Axonemal outer dynein arm (ODA) motors generate force for ciliary beating. Each HC of the axonemal dynein consists of an N‐terminal tail domain followed by the motor domain. This includes six AAA motifs (named AAA1–AAA6), with a microtubule‐binding domain (MTBD) connected to AAA4 by a coiled‐coil stalk, similar to its homolog cytoplasmic dynein. We analyzed three states of the ODA during the power stroke cycle using in situ cryo‐electron tomography, subtomogram averaging, and classification.

We thus have obtained an apo state, depicting the post‐PS conformation from a nucleotide‐free dataset. Our analysis shows that in the absence of ATP, all dynein linkers interact with the AAA3/AAA4 domains, indicating that interactions with the adjacent microtubule doublet B‐tubule direct dynein orientation. The tomographic map suggests that the γ linker is in a Post‐2 conformation, which was observed in neither MTBS1 nor MTBS2. In situ all three linkers appear to be in a Post‐2 conformation. MTBS1 fits worse than the MTBS2 model, which has the β and α homolog linker in a Post‐2 conformation. To optimize the fitting of the MTBS2 to the cryo‐ET map, we performed rigid body fitting and real‐space refinement of individual parts of the structure by Coot. Step 1 is the translation and rotation of the γ dynein head including the MTBD. The linker of the γ‐HC changes from a Post‐1 conformation to a Post‐2 conformation (Movie EV2). In addition, the stalk of the α‐HC adapts to a more straight conformation by a 1 nm distal movement of the MTBD. The resulting MTBS3 structure is shown in Fig 3F–M. Through this remodeling, the cross‐correlation score between the 20 Å filtered MTBS2 and MTBS3 structures and the cryo‐ET map increased from 0.6797 to 0.8402 (Movie EV3). In the post‐PS conformation, the stalks are upright and extended, maintaining a certain distance between two MTDs.

> MLSSKYSKRIAWMKTTICDSLQLKDMIVEESFQYEKNKNLLEQFLSGEGLNKIFAYYQVQEQAQNDDIKDTGAQDPVLFFTTGDLEKIQDKAVWFLRITNPADDKKKASQQDGNDNDIIFGEITPNTVPMLNALMESVYSRQIDHIITEKIQFWGVAEEEQVLEFQQHSNKFSSEVREAINLMSPGTEHFKLDYEAISGLSESEKMQHYEMKFNEWINLISSQLNDDSEVRKDEKDAGPATELIYWRSRMQKITNWSEQLKSKDFQIVKASLQRHKNHDNQRPRGDESLSKLMMEYNRLDLLLTDKLNEAKDNVKYLTTLEKFIEPLYNGTPQQIIDTLPALMNAIKMIHTIARFYNTTDKMTGLFIKITNQMIKNCKDRILNKKDNGDNPSLYKMIWEQDPAELIEVLGSCIKLYCEYKKCYNDTKEKVADMPKGKTFDFSDAQIFGKFDTFVRRLQKLIEIFSNIQQFNALAKHNLEGMDVLTNKFKKIIDDFKKKGHNLLDTANNKFDRDWVEFNVEISHLDGELQNFIDNNFNRFRNIEYSLKLLHKFQSTIKRDSLKHNLTSRYNAILHNYATELDTIQRVFQDQKSNPPLVRNMPPEAGKIIWARHLFQKITGPINIFPENVINSTEIRRYYGSYNTLGKQLTIYEMWFYQDWVNKIEQSKAALQATLIVRHDENKKLYVNFDLEIMQLIREAKCLDRQGIEIPESARIILLQEDKFKTYYNELLYALKEYERINSKIKPICKNLLLPHIEDLDLKLRPGMVTLTWTSMNIESYLYYVHQGLKKLEQLIINVNDIIENRIENNLKTVSKVVLVHLPQDTKPLSLDSFVQLQEEYINSKTDFLTSKNVEVERAVDDLLQTIMLYPLDPHVDPVLPEETKRIKRYYFWYFYQALLNSTQNSLNAMKYRVCGKKIPGANTLQNLKPFFQVEVQLNGDKVTLNPSLQEIQKSINRAATAVLRCSKHLYNWDQQNKDSTDKATFYDMIACDKEIVKVILLLTGSIQGTKNKVNEFLSGFTKFEWLCKESIQESIKKFSKNGPTLQNYEDQLKKFSQIEEEIEKIVPTYKIGAMELMTHNICTSLSTWAKEWKLQYSQDLHKRARQLLDSLTEQTKMLSTKLSKPVKDIDSLGYVMETLEQIRKEQAEIDMKFNPVQEMYSLLDNYLPGGITDKDEMDARSLLRRNWDILIQQAEIKGKEYQHKQAIYLKELKQSIKDFTNQVSIFRRDYEKNGPMVEGISPAEAMERLRRFEDEYDVKYQMYKINARGENLFGLQNQKYPELEKTDAEIKNLNKLYNLYDSVIKNIQQFKEKSWQDVSKDDLAKMEEDAGKYGEQCSRLPKDLKEWQAYRDLKNYIDSLREQLPLIISLKKPSIMPRHWEKIKEITNTKLNYENPDQFYIEEIMGAKLLDFREDIEDITESADKQLKIRTGLDEINLYWNDMQFQFGIWGKRDVPCMLNGLIVGTILERLEEDQLQLSTFNSQRHVTPFKAEVENLIRTFSDVNDTLDMWVKVQKLWTSLEPVFTGGDIARQMPLQAKQFQGIDKNWMKIMEKAVETKKVIPCCQNDMLKDFLPDLNRKLEDCQKMLEAYLEGKRKKFPRFYFVSNPTLLKILSQGSEPTSIQEDFEKLFDAITKVTFESAKDKKNPALKQITQIQQVIGRNEENISLTGYYVKCEGNIEDWLKKLEQNMQQTLKDIASAAAQQVFQVGLKEFVSSQASQIALLGLQILWTSKVNEGLERLSRNERNAMDIKRNEIKEHMNILSSMCLEDLNGAVERTKVETLVTIQVHQKDISMDLKCKDVNDFEWQKQTRIAWKTDIDECIISITDWDSPYSYEFLGAKERLCITPLTDRCYITLAQAMSMYYGGAPAGPAGTGKTETVKDLGRTLGVFVVVTNCSDQHRYRDMAKIFKGLVQSGLWGCFDEFNRIDLEVLSVVAMQVESITTARKQHMKKFMFPEEEIEIELIPTVSYFITMNPGYAGRQELPENLKVLFRGVSMMVPDREIIIKVKLASVGYLQIDLLAKKFNVLYRLCEEQLSKQRHYDFGLRNILSVLRTAGNTKRQEIKSDEEMLLMRSLRDMNLSKLVADDIPLFNGLLADIFPKLKEVPKKLYPDVEKKIPEEINAESYLINTPSFQLKIIQLYETCLVRHGFMLVGPTGSGKSTIMKILTEVLTKLGSPHKIVIMNPKAITAEQMYGVKSEISDDWIPGVFSTIWAKSNNRALKHTTWITCDGPVDAIWIENLNTVLDDNKILTLANGERIAMTENCKVVFEVENLNNASPATVSRCGQVYVSPTDLGYEAVIEGWIRNRKASGRAEESDKLGNILRKYLINMRFIELQSKECKEPMMDTSPVISVINILNLLTGCLQYFVQTQRTLSEQEYEKFIVYSMAWAIGGIYEAQDRVRFHELLLAKNAPIPQKGKENETVFDYYVSQDYLDWKICSPEEWVPPQSLQFSQLLLPTLDSFRAEMLLNFILTQPKSHTCSNSALLIGGSGTAKTSSVLLYCNKFDPQKMLFKRTNFSSATSPFMFQSTIEAECDFKVGKEFAPPGNKMMTIFIDDMSMPFVNKWGDQITLELVRQLIETGGFYMLDKTQRGNQRKMKNLQYIGAMNHPGGGRNDIPNRLKRQFFIFNMILPLSIEGIYGPIIKHMFKQKYFSDSTYKVIESLTSATIALWNKVKSTMLPTPAKFHYVFNMRELSRIFKGILTCKKDTINDAPKSMKIKPELFLVGLWRHEAERVLADKLVNNKDKDTVMGYIQEVSLESFSQIENEILEKYSSEKTFLFCDFLRPDVINEDGIIEEEAPKIYEAIDSLTELRKRCNFLLSFYNDRNPSKKMPLVLFDDALKHLLRISRIIRQPRSSGLLVGVGGSGKQSLTRLAGFIGKNLIQQIIVTKTYSDKDLKEDIKKGFDDAGHLGKQVTFLMTDSEVKKEEFLEYINMVLSTGEIPNLLAKDEREVWLGDISQAYCKEKNLGNIDPPQSELWTYFVDRVRDNFHIMLCFSPVGQKFRERARKFPALFNECTIDWFLPWPEEALVSVAETFIKNFDKLDTKEETKQELMKHMGNVHLMVNEICDEYYQKMRRQVYVTPKSFLSYLNSYKTLYIEKYDELDQQEESFKIGLNKIQEATITINQMEISLKEEEIQLNEATEKTNQLLANLDKESKKANQKGEEVAATNKQCEIQAEQISKEKEEAERELEAALPALRRAQEAVDSIESKDIVELKANKKPLDIIKYIMDAVLVFFKARLIPIQIEERVFNKKEGKAVLFLKESYDESGIQTLGDMNFMKKLKEFEKDSINEETIELLEPYLNQSEDWFNDTFATKASKAAAGILKWAFAIYEYHQKSKIVKPKRIQVAIAEGRQAIALKELEKAREDLAQIQAYIKNLKDVYTKQMEEKNELEMKAAKTKKKINTARTLITSLSGEKDRWGKGAQDISDQKRKLVGNVSLSTAFISYCGPFNAEYRNKLAQQRFVVDMKKRGVPVTPGLELTSFLIDDATIGEWNLQGLPKDDLSIQNGIMVTNSARYPLFIDPQGQGQNWIRNKLSASIIPERCITTLSHPKFKDMFLKYCMESGLTLIVENIENEVDPMMDPVLERQIIVKGKTQFVNVAGTEMELSKEFKLFMTCRLANPSFSPELSAKTTIIDFTVTQSGLEQQLLGKVISKEQKALEDSLNQLLADVNQNQKDLQRLDKNLLERLINSQGNLLDDTELMDVLNNTKTQAKEVAAKLIDAEIKTKEINEKREQYRPVAIRGSAIYFTMIEVSLVNWMYNSSLEQFLKLFIESIDLSEKAQLPSNRVKNIISFLTFHVYRYVNRGLFEKDKITFILMMAFKILTTAGTISSGDVSLFLKSGDALDIKSERQKQISYLEDNQWLNILALSKHTFSGQTLPFFKELPDLISRSENQWRNWIDKNDPENFPIPDFAESINQEKEIGSFISLCLVRSLRNDRTLIATQNFISNVLGKEFTDPISYPIEGIWQESSNMDPVLFLLSAGADPTSSIDELAKKKKKFPCEKVSMGEGQERVARQVIMKGFVEGGWVILQNCHLGLKFMEEIETLVSPINQIHEDFRLWITCEQHPKFPLGLLQKTLKVTNEPPKGLKAGLYKTFTTIITQEFIDKVDHSNWRSLIFTICFLHSIVIERKKFGPLGWCVPYEYNYSDLEASLLYIEKYLTNLMSTPQPNSHNLPISMNVVRYMICEVQYGGRITDDLDRELFITYGETYLKDGIFGNDYFFYDIMVDGSGQKFKYRIPQNPSAELIKYQEYIAKVPTVDNPEVFGLHSNADLTFRLKESKEMINTVMETRPKDSSVGGGKTREEIVQDKAKDMLKNLPPDYNDVEVRELVSKLGGPNPKTSTERGMTVPLNIFLYQEVTRMQRVIGLVRKTLQDTILAIDGQIIMTPEILEAINAIYDAKVPNSWLYDPSGAEISWLLPNLGSWSTSLSDRNKQLNDWLRSGQRPILFWLTGFFNPQGFLTGMKQEVTRNHKKKDGKGGEAWSLDDVVYSTTVKEREKEKDIEQPPAEGVYIKGLYLEGCKWSKNGLDDSDPKKIFADLPILHVSAINKKKTNEQDRMSNTYLCPVYKYPKRTDKYLIFRVGLPCEGSNNPSHWKLRGVALLCSTE;> MGDHSQKDSPEDFIINRLSQALGIQKEKIKKSLETQQDDKGEVTNKDEFQGFIQQDNSTNILWVSGQSEKCTFYYGQLPPIDKFKKKGIAVIKLGLHKLTNENVAKDVVVVEITNNLLEHLNSVFNEIMSPVMQNPLNQQGWTDLVAKDLMEKFNNYVAQVYVLLGQIKGKTMLPLPSHKLTSSDTTPDKDKAHVFEGSIITWTKQIKNVLKLEPEQLLKYGNDPGPLAEIEFWQNKRDNLNLIDSQLKSVEVQNILHFLDNNKSTYTTPFTKLQAEVKKARLEANENYRYLFTLKDLFSKLQESQPSDFPTLYELFIPIMHTILLIYNKSKTYNQPPRLVVLIREICNAIISNAQAFVDKDTIFSLIDSKETTEACDKLQVTLDVCSKFKDAYFEYKAKAGGNWKLTSNALFVRLDSFLERCQDILHLTNTIVQFNKLEKIELGGTKGKTLTESIAQIFKEFEEAVQAFTSVSYDIMNIAEKKFDDDFYEFRSKIKELERRLASVITQGFDDYDTIYGRFKLLDNFEGLLTRPIIADELEKKHIVLLEMYKQDLKQVQSIFLEGKQFVDSMHENAPLFLNMPPIAGALTWCKSLRDRIQEPIEKLAQLGQGITEREEYKDVQKLYTSITKSIKDYEDQKILSWEKEVEDSSQDKLKQTLLCKDENDLIKVNFDPSLVRLLKEVKYFLLLRLEVPTTAKDIYTKAETYRTQIVALDMIVDNYNHIKTCLLPVEEPLVKKKIQDMEEEVKPGIEEIRWKSTNIDQFISKSKSIVDQLFETVNKMKDSLQKIHKSLANFNVKIIERKNRPMSPDDYDQFLKAIFSNKLTIVKDNGNQIQKLVKEVLDAVKADKKQNSWKNYNDYVNVIVIEGISTAIQTALLHLNEQINPVFIKRNDISPLFDIRLELGQSGIQFDPEIGESSNQLTVRNTIRNWINDFFNIAGTIQRLDTTMPGDFLQEIRSFFEIKQCLAMITQNLEWIENECNQFRARFDTYSYLWTEDEQISFNRFLDENEPKDEDGKGGDDDEGENTEKQNPLLKGCRAKIPNLDLFDEKITHLKAIQQEISRIKTPEDISWLRINLQPMKTALDARVTRWIRVYTDFLVNQFRTTQKNLLDFIEKTKDGIKKNPADHENLHDKKLLMSVMKVISDVKDVEPRREGIITRMKEMVTKLKKHNVPITEKGTDDPLQQIDNANSNFIEIYGRVFKVKADIIPLQAEETQNIKRDLDIFMKEVESFRKEFMQKLPFDYTESMGYENINNAYDTIMVYYHKLTAIEGRALEYNNLEKLFELQKSNYKQLKDCMNDLKNLKTMWDAIALIHFQYNDWKTKPWRQIKADILLDTNKTLGTQIKNLPKEIRNFKGYNVIVEKVKNMGTVLPLVSALHSEFMEDRHWSQLKQITGTVFDHNSLSFYFEDILALNLYKYENTVNEIVDVAQKEAKIEKKLKNIEQWWSKQVFEFTEYKETKTFASLDNMMEVLDQHSLDLMGMKSQGKYVEFFYDRVEDWREKLGRVDVVVNEWLKVQKNWKILYNIFLLSEDIRMQLPEDTKVFEGVDKEFKDMMSEVSANPSVVEACTIERRDVLVGWSQAIKKCEKALNDYLEQKKKSFPRFYFLSNQSLLTILSNGQNAPKVCEYLGDCFDGLKTLTFEPPANPAETSKVGIGMISKDDEKVPFSSKFICEGAVEHWLLNLEFRMRETLQEILEGAKNTADLWDSGDKPREEWVEGYNAQIALLTTTIVWTEDVGRAFEDLAGGSETAMKECQKLIEVRLENLIKKVRGDLHILERWKIINIITIDVHSRDVVEKFVIQKVSEAESFAWLSQLKFYWENKPDSDMHLRQTLRFPWEKDKNKNKCIIRIVDWFRFYSYEYIGNAIRLVITPLTDRCYITLTQALNLTMGGAPAGPAGTGKTETTKDLGRAIGIPVMVFNCSDQMNKDSMAQIFMGLSQSGAWGCFDEFNRISIEVLSVVSTQVKCVLDALKEKKTKFSFVEEGEIQLQDTVGFFITMNPGYAGRTELPENLKALFRSCAMVVPDLALICENMLMSEGFTMARVLSRKFVSLYMLSRELLSKQKHYDWGLRAVKSVLRQAGKLKRGDPDMPEDPLLMRALRDFNMPKIVTDDKVIFRRLIGDLFPKLDPPTKQNPELKKIVQDTTKKDMGLVAEELFVTKVVQLAEILEVRHCCFVIGPPGSGKTCVWKTLIKSYINSGEDAEYDTLNPKAVTSDELFGAYTKTKEWKNGVIAVIMKNQVKNEEKYKATHMHKWSVLDGDIDPEWIESLNTVMDDNKVLTLVSNDRIFLTPQMRLIFEISNLRNATPATVSRAGVLFINETDIGWMPYMNSWLERSQINILKQQKEMANMPEYPVIDDVAKSVFYRCFQSYFEQNIDVHDKNRVRHICPMVDIAMIQTICTILDALLIQHLPKLKQMKEEDEKQALEAFFIFAGLWAIGGPVGGGQDDSKDMKEFNTVWKGAAKVKFPEQGLCYDYYYDINENKWNTWKVEDYLPNDQPLFSKIYVATIHTTRLRYMIDIHLQRRKPILFIGSAGTGKTAVVRDYLNSTRPEQVSHKTINFSSFTDSLALQKNIESMVEKKNGRNYGSATNKVLICFIDDFNMPYVDKYGTQSPIQLLRLILDYGSIFNREQLEERKFLQDLLFFGCLNQKSGSFTVDLRLQRNFSVFSMYTPSSDVIKTIFGSILNAHLSTIDDKAQKMAFKLVEATYFTFDKILKNTTAFAPSAKRFHYQFNFRELARVCEGICRTTPGQYSGGDQGKLVRLWAHEMKRTFEDRFIANEHVEFFRRYLTEAISKCIGEFPETENPIAEPLIFTGFVAAHQGLDQQYTQCTIPVLKRVLDDKLEEYNEVKAQMNLVLFQQAMEHVSRICRILDMPGNNALLVGVGGSGKQSLCRLSTFINGFEIDQLVVTASFTINDLRNNLQEIYKKIAKPNSIARVFMITDSQIKEEQFLIPINDMLNSGWIFDLFPKEDMDSLVSGVRNEAKGEGVDVNNLTALTSYFLDKIRKNLKVVLCFSPVGDTMRIRSRKFPGIINNTSIDWFHPWPHEALIDVAFRFLEEIEFPTEEIRQSISLNMAKVHSSIDTANEKFLKLERRYNYTTPKSFLELIDFYKKLLTEKRETIQRQIQRYEMGLNILAETQNKVQGLQEELKVKMVEVNKQREETDILIEKVGKESALAEEEQTIANAEEEKTNVAAAEAEKISKEATEALAEALPALRSAEAAVDCLKKPHVTEMKNLGSPPAGVIVTARVVLILFNQGITLNDPDEKVWKKAVTFMNNPQAFIDKVKSFDGENIEPNIIEQSNKIIQDPSKKFNEKDMAGQSYAASKLCAWAVNIVTFNKIFKQVKPLQDAQKQANEILEEKKKELAIVKQRVAELNARVNSLKRQLEEAEARKMIVEQDAARCQSRLSAAENLVNGLAGENKRWTQNVKFLKENIKSMIGDSLLASAFVSYIGAFSAKLRLELWKNTWLPDIIEKGIPITEGIEPLKILTTEAIKSKWKNEGLPADPMSLENAAIITACARWPLIIDPQLQGSTWIRGKQGENLTTISLSQPKWLGALTSSISSGRAVLIEGIQQEIDATLDPLLQRAVKKNGNQLQLEIGGDPIDYDPNFKLFLMTKLINPHFRPEIAAQCTIINFIVTESGLEEQFIAMVVNIEKNELEMAKQDLVKKQNEYAVTLDKLESDLLQSLSEADPATILDNTELIQNLDKTKKTTIEITEQQQKAKVTEAEINIQREHYRVVAAEGSMLYFLVISLSVMDHMYQYSLESFITFFFKAINRTTVRDENRIPTLILNIRQTIYQWISRGLFEKHKLIFLTLIVFRLMQKKIIDVAYEVAEMDFLIKCPARPGVENTLDWLPNISWDQIQGLINLEEFRNFAHQLEKEAPNRFKDWYNELQPEDQKLPLDWKRLDSMPFKKLLVLRCLRPDRMTISLNNFIRAVLPQGDAFVEMDQKLAFSEILESVINEDSESTIPIFFILSPGSDPVKEVEKIAKKKRIEPGKNFFNIALGQGQDEIARRRIEEGNKEGHWVMLQNIHLMPTWLIELEKILDSYSGEAGGGNSEFRLFLSAEPSTGIPIGILDRSIKLTNEPPAGLKANMKRAWTYFSKEEIEDKDPKIKSILFALCFFHSTLIERRRFGPKGWNMSYPFNMGDLRDSYLVMNRYMEQNQGGKVPFNDLIYIFGEIMYGGHIVDDWDRRLCNSYLFNTMHEQLFDELELFPYIEGKGLSFKVPGQNPYEKYIEHIETSLKQETPLAYGLHPNAEIGFRTDQCKTLFNTLLELMPKEQSRDEKSSDIKSSNEMASDLIKQLLEDSELKNKIFNMEEIKNKIDAENKGPYQNVFLQEIEYMNALLSEIVKDLEEIGQGLSGLLTVSENMEMIIESIALSRVPASWQKLAYPSKRGLQSWLANLFQRIEQLNIFRDDPYSIPRVVMISRFFNPQSFLTAIMQVISRAKAYELNKLYIQTEITKRSIEEIEGAAKEGAYVYGFILEGARWDYQLGQLEESKPKEMFSVLPVTYCKAIPLPPEGKEDKSLYQCPVYKTEDRGNTYVFTAQLKTRFPPRKWILAGVAIIMDVEGVSDEVKKDKK;> MPQPLVWTQLKQTGTTQPTARSGHTIITVGKTHIMFGGLDNDKNNYKDGKIAPNNQVFTLKLTQNNCEWRQIACQGDVPLPRCYHASCAISADKMLVFGGSYTSNLRFNDTYILKTTSYQWSKPANQISGGEPKNAESKIGAPQPRYGHSATFFEGKVYIFGGHGGINYQRLAFNDLYVLETENFEWTRLEPKGNPPDPRGGHSAAMMANKPQLMIFGGWSFTSQYSNIMIYDIEKDEWVDPEIAHEIPKWNLSGIMAPSIPSWKYFIFGGSVGSFEEGGNRTNSRFVDDSFVLDIDTLSWSSINLEADETSKAVCKPRPRESASIFYDSGESRAIVFGGWANNWLNDLWALNVSTITGPPYAIFSIKPALGPLTGKTKVLIEGDGFKDTQNISVKFSGGKLEKEVNGTFVNEKEISCETPTFDYPRSVEVTVCMNKGDYTITKSAFTYYLNTKADKTIAYGPGLLTENLIGVQTTIVIQARNKNDQNRESGSDEFVVTIRNPAKIKKEEEVKEGDKANTKNTIKEDEEEEGEDEEENKKKKEAEKAAAEKAAAEKAAEEEQGEAVDPSLVPFNIVDNDDGSYFIQFTSEEEAVLEIDIKFKDENNELHSIRGNPFRCGFVKGSKPNNNDLTGSAVMNYISKQLKDIQEFIENTKENIEIRNKNIRENVSELINVMINLEKVRVKNDDDVLTLDTVEEMLNFLKKKDFGKDSDIKKCKKLQEEWKNLAKMAQAVKKDIQNPVKTESDKTKENIKKFEEITLKEYANSLKKESFFIYKTGVSESFKRIGEVKQKVDEFEVQLNQYEDFARMFEFPDAVIGSKKLMEQIRTDVSSVEKLWVRIEISEKTMDEYKKMKWGSINSMDMEDEIKKLRKALTDLRGIDKRSNAFIGITEELKKWATFLPLLGELKDPSMNSEDGRHWKKLKDLVKKEFDVSQELMLEIIWDLKLFDYKDGIEEITDQAKQELKMEKALKKIIDFWRDIEFELVQHKNTDIHTLKMSEENFETLEDHQLQINNMLLSKYVAYFEKEVEKWKYDLGSVYDVVQLLLEVQKTWSFLENLFIQSEEVKRELPNESAQFVGIDKDMKEIMQKGCDIKNCLKFCTIEGMLKRLENIQAQLKVCEKALNEFLDSKRRAFPRFYFVSVNDLLDILSNGNSPAKINRHMSKIFQAIDNLQLKEDSSGGRPTALKMISCVGTEEVDFSSPRLLQGKVESYLKDVIDTMIGTLKSVANSSFKNFQSMTRKEWLKSDPSQITLLVNNIIWSKAVEDCFLKLQSGDINAMKLFLDESIKQLTELIGMVQGDLSKPLRQKIMCLITIDTHSRDVVHRLINEHVRKAEEFQWQSQLKFYWVDNDAKIKIADARFVYNYEYLGNGPRLVITPLTDRIYVTATQALHLKMGCAPAGPAGTGKTETTKDLANALAKACYVFNCSSEMNYESMGNIYKGLASSGCWGCFDEFNRLLPEVLSVCSVQFKAVTDAIKQNVERFIIEGDEISLDPTCGVFITMNPGYLGRAELPEGLKALFRPITVVVPDLELICENMLMAEGFIEAKILAKKFVTLYMLCRDLLSKQLHYDWGLRAIKSVLVVAGGFKRSEPEIAEQALLMRALRDFNIPKIAFQDLYVFHGLLGDLFPGINIKPKKDLDFEKIITDVCIENKLDPDPEFVLKVVQLSELLAIRHCVFVMGPPGAGKSTTWKILAKAQDKTNKKTTLIDIDPKVVSTKDFYGYNLPSKEWKDGLFSKMLRSLAEQPDTNPKWICLDGDLDANWIESMNSVMDDNKILTLANNERIPLKPHMRALFEIRDLRFATPATVSRAGILYISDEVGYQWRSYVKSWIKQEFSQDQEMSKNLDTLFGKYVPDTLDHIKKHCRFLVPVSPISQVISICKSLQTLLKGDVKNLEYLFVYALIWAIGGALAEKDSIDYRKDFSTWWKGAWKTAVKFPSKGTIFDYYVDQSGDSSKFVEWSKRLENKEFDPQVETMGNITVNTIETLATTEFIKSYLMVKHPSLLIGNSGCGKTQLAKGILKEIVQAKPENYAYQLINFNYYTDSTYLQGQIEQTLEKKAGRQYGPPGKVQLIYFIDDLNMPQLDAYDTQTAIALLRQLADYGHFYDVSKLALKDIINTQVLAAMNPSAGSFFVNPRYQRHFWTISIPFPDNESLSLIYITFLNGHLKRFKSTIQEYSNIIVRASLMLHQAVTQNFRKTAINFHYEFNLRHMSNVFQGLLLSDPNKFTEPDKLIKLWIHECERTYGDRLVSTDNLKTYKENIFDIVKKSFSKFNFSRYFGNNPENLIYCNFIAGINSDRFYDQMPNNEMEKHISEALKEYNDNNAFMGLVLFEDAMKHVCRICRIVLPSSGHALLVGVGGSGKQSLSKLASFIMGYTTFSITISATYSMVDLRNDLQQLYFKCGPKEEGILFLFTEGQITNERFLVYINDLLSSGEIAELYTLDEKEAMINQVRAKVKGEGKPDTRENCWNWFIDQVKKNLHMAICFSPVGDMRRRARQFPALVNCTVIDWFQPWPYEALFNVAKSFLEPVDLGDDKVREAVVKFMPFSFTLVNDLGLKLLEQERRYAYTTPKSFLELISLFTNMLAQKRESLERNKERYETGLVKLKETAEQVAIIEVEVKEKQVEAEAKKKEADAFAEVVGREKDKVEKENSKATIEADKCGLIKQNVEAQKSSTQQDLDAAQPLVEQAKSALNSISKKDFQQAKSFASPPAGVPEVFAATIYLLAGYFNEAIEIDKNKKPKDVSWKSSLKLMKSPEEFMEKLLNFKDVVDANQVPAANVNIVKNQYLNMPSFTPEQMASKSAAAKGICSWVVNIVKYYDVIQDVEPKRKALKEATEQLEEATVKLNEVEEVVRKLNEELNKLKAENDKAIAERNAAISEAERCARRLNLAQRLVTALSSENERWGKSIIQLEDQLKLMVGDVLVASSFVSYSGPFNKKFRNIMINQNFMKFMKEHTIPMSPDPNPIKILTDESTIALWNKQKLPSDSVSIENGTILTNSARYPLMIDPQLQGITWIREKEKANNLKILRLGSKNINRDLELSIENGYSAIIENMNERIDAILMPIIARSFIKRGKNKIIKFAGKDLILHPNFKLFLHTKLSNPHYPPEIQAEAALINFTVTEAGLGDQLLSLVVARERPDLAKMKIELITQQNDFKIKLKDLEDELLYKLANAKGDILDDIELIENLEYSKKLSVEIAEKVAAAKITEAKINETSENYRPAASRGALFYFLLSDLSKVHSFYKYSLESFIVVINRAIDAISENKIYGKTTMVPYGDETYASNQHEKEEEEEEEEHQQAQQQQNQEEQQEQKDEENKGPVEEEQPEGENKGPVEEEGAEGQNEGPVEEENAENQEGEGEEEGEKQQKAKDSDEPMSPRSLKKRVDELIESLTYTAYQTTRRGLFESHKLIVAAMLCLRVLLRSEELNSDEVDHLIIGKVDVNPTPMPDALKSFLNDNIWAACKALETIHQFQGFCQSLETDVLQWKKWYSEEKAETADLPKAFKELSKFHRLLLLRALRPDRLPSALSQFVHDKMGERYIEQPPFNIFETFQETSKTVPIFFVLFPGVDPTPDVERVAATFDVSANNGRFINISMGQGQEDRAKKALFDCAQKGHWIMLQNVHLMQSWLYGLNGLEGFLESVFASPKTHPNFRVFISSEPPNVLLPLMQIIPESILQGSLKIANEAPQYLKANLRRAYNKFDQEFLDKCDKKPTEFKSCLFALCFFHSLMLGRKKFGTQGWSRVYNFNDGDLTICADVLYNYLSKYDQVPWDDLRYIFGEIMYGGHITDDWDRRTNRTYLKVLIRSELLQQNFNLAPQFKSPDPSKFDYEAYRKYIEEKLPIESPQMFGMHPNAEIGYLTQTCDQVFNTILEVQGGSSGGGASKKDDGVMVTLTDFKTRCPHDFNMLLIEEKVKEKTPYIVVCLQECERMNGLLKEIKTSLEDLRLGLTGALNMTDAMESLQQSLSFNKVPDTWEKKAYFSKKPLSSWFADLIERNIQLQEWCKELVTPTSLCISYLFNPMSYLTAIMQFTARAQGLPLDGITIQTNVTAMKGPEDVVNPAENGAYIHGLFLEGAAWEIGGQGQDGYLIEQKPKELHPKMPVINAVAVPLDKKKKNGQYDCPTYVTSARGQTFVFTANLNMESDDSDPNKWILSGTCMLMSDD;> MPPKQTKVVASRKTVMPISRAGRAQIRRKDSNTQNNMNDQGMEDEEIDQQREGMKNQYEQLTAQELNEDMPSKMLEPKNPQAPKNITVYDYYTRKFKTDELVDQMIVHFSMDGDYIWKESNEYKTQEEIRDTKKALIKEAMRKQESEEPGANHDEEAIKQTLRNKFNYNTRECQTINPSIRERGVSTEPPPSDTICGNITQWEIFDAYYAEIMKDHQIENKKKKEVDQDKKQDQSMYSTSFKRCCKIMERMVVQNDQEDKYHDYRYYWSQGDNLEAGKNEGHLLPIWRFSNEKQRKKNVTSICWNPLYPDLFAVSLGSYDFTKQRMGLICLYSLKNTTHPEYAFNCEAGVMCLDFHPKSAALLAVGLYDGTVLVYDIRNKHKKPIYQSTVRNQKHTDPVWQVKWNPDTSKNYNFYSISSDGRVMNWILMKNKLEPEEVILLRLVGKNEEESTLIGLACGLCFDFNKFEPHIFLVGTEEGKIHKCSRAYSGQYQETYNGHLLAVYKVKWNNFHPRTFISASADWTVRIWDSKYTSQIICFDLSMMVVDAVWAPYSSTVFACATMDKVQVYDLNVDKLNKLAEQKIVKQPKLTNLSFNYKDPILLVGDSHGGVTLVKLSPNLCKSGPEIKQTEDKKAMEEFKNVKIEDYEREKMENLLA;> MAEYFTYSKKRKEFNNPINFQDTETRYGGIQNQVVNINQYVQRNPNFIDLDNIAELSEHSVNTERVKTGDRGMSHKEGGWPGNVDPNEAQETGRFKKRIEKDTSFPQAVKDLKEGVEKCIYQNNQIDLLEEYFEGETSEHVVENLSSKTLMLFKDEKEICKRSVSEISWHPEGPTKVAVSYAIMRFQQMPEKMPTQAYVWDLLNPNSPEIKLMSPSAVTNISYNQKIPDQIGGGCYNGLLAVWDGRKGENPIMISPVENSHYEPVTHFHWLMSKTGSECVTTSTDGKVMWWDTRKFEAGPVEKLNIIEGLGENEEIIGGTALEYNVEAGPSKFLIGTESGSILTANKKLKKPVEITTRYGLDQGRHLGPVYSINRSNQNPKYFLSVGDWSCKIWVEDLKTPIIRTKYHGSYLSDGCWSPTRSGAFFLVRRDGWMDVWDYYYRQNEIAFSHKVSDSPLTCIKINQTGGAYHNSGKLCAIGDQDGTVTILELCDSLYTMQPKEKDIINEMFEREYRKEKNLETIKKQQELAKRQVQKDMGSQKEKWEKKKLEMIETAEASFHENLAKNPVNEEEFNELDSPSEKRKKTNQNQGREQEEQSREEQEASGNFNQQQQQQQEEEQQQEGEQQHHQNQEHQNGQGHENGQEEGEENGEEGNQQENEGQEENEQQQE;> MAQDINADDQLKQLSALEGANGYVIFNESGIPLKRHEKSISHEKAVHIAALVSDLWNVSKKVIQRDLKTPENDIEVIRLRTKHSYEYIITQSGDFTMLAIQLCGKAIEEAKKAAAAAAAAAVVQEENKEKEKK;> MIYKTSKEIQKSDQRIIQQRVENSIINNQIYQKSLKRKTSKRKVRHQANKKNFQKEMSEVEDTLNRIKTHKTVLGYLIVNSEGGVVRGAFKDEEESKNIANSIPLLTKKARSVVRDLDPTNDLVFLRIQTKLNEIMVAPDDEFSLIVIQTKGEKRDEND;> MSHLDKVQPVIKNSDMSVEMQKEVEEVAKKAIDYCNTDKEIATFIKDDFRSRYHGTWHCIVGRNFGSFVTFERSYYIYLYVGQLAILLFKTG;> MEQEKAVTDMDINELRKLMIGKAIINSSDMQGDLLQEAQDVIQSGIENNSAPVLNIEAACKYIKENLDKKFGPTWQCIIGEGYAYDVTVQNNTLLFMFYNGNLAVLIFKS;> QQYKTFMGARVLWPPECADDILEGAIRETQDALKKFEIAREGQKIAEHLKKYMDDHFDPYWHVFFGKNFGCQAVHNKNRFIYFYIEKTAFLMYQT;> MGDHANEQIIDMPENSEMKSMKNDAFSQAKFAVENYKFENKISSHIKKFFDEKYGPNWHCVVGKHFNAYVSYDSKNFIFFYEGQLAILLYRKG;> MSDSDSDEGRVVEEPLPPHIIRFNDMAQHLLKKVIRQADVLIKENPQGLEKDIALNLVKFVKSQPEFKIGDGEWQCIIGKNFGCSLTFDANVLAFFDLLPSRKSILLFKSG;> MNHEPEVKATDMEEDMIKRVKEIAINAVKEYKQEKQIAHYIKYEFDKIDGYGWNCIVGRNFGSHIIHQTKKYIFFKINELCLLLWKA;> MGDTDKEYISEEVQKAIDDSVKQVFGIKDDSSQVTITYNKDKVNLWTQQIIDYTIRGLNKLGKHFKYCVTAILQQTNHAGISVQITAYQDTNTDGSLIQCYEINDIYAIVSVFAMAV;> MKGTYLYLNIYKRKREASLITLNYIKNRFYPSKIQKIIKELFEDRLKGVEYDPNNANQLSERLVLELREKIKRGKVPRYKIGVQVVFGEIKGQGLRIASKCLWDVQNDNYASYTYTSEKVYCTGIVFGCYFE;> MSKKQKKEITTTVTSEDHFMTFYNENNKKLIVVDVYPGWSGPCTAMYPTYNQLMISIDDFEKRIDILLLDQDKLVTYKNDKFHATCQPKFLFISEGKIIDEVLGTNIPVFIEKVNKYIPLSY;> MSKGTTCQKAIVNWEAANPGKNPSEAEEIKLIFQIPPIEKMDGPVLNTLTKCKKLSLSSNSIDKMISLNMLRNLEILSLSRNVIKKISGLEDIGGTLRQLWLSYNFIEKLDGLNNCSVLQTLYIGNNRIKNWEELDKLKDLPELENVLFYGNPIYEQVKEDPKLIVLKKLPTLKNVDGYIIDDSVLEKVKQIADIPISAKQL;> MASEVMNLSEEDIQFCQKAFSDYDEDGLGAIKVSDLKLALENIGCSLSENDLFKMISEVDEKNTGLIKFSDFLNIYYKQKYANLGDDDQDLVDAFVAMGGNADTTGSVDANRLIQIVKEEFEMTIDIVGLIREIDKDGSGEIEYEEFKLLLKSGFANEGN5-(1H-benzotriazol-6-yl)-1,3,4-thiadiazol-2-amine 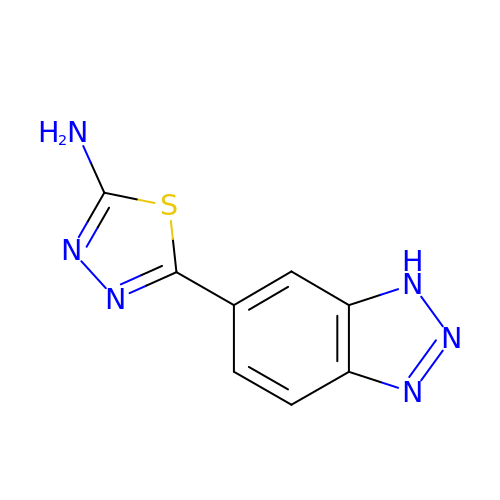| C8 H6 N6 S | QEDRDOHUKCLXOP-UHFFFAOYSA-N> MGWGGGGGCTPRPPIHQQPPERRVVTVVFLGLLLDLLAFTLLLPLLPGLLESHGRAHDPLYGSWQGGVDWFATAIGMPVEKRYNSVLFGGLIGSAFSVLQFLCAPLTGATSDCLGRRPVMLLCLMGVATSYAVWATSRSFAAFLASRLIGGISKGNVSLSTAIVADLGSPLARSQGMAVIGVAFSLGFTLGPMLGASLPLEMAPWFALLFAASDLLFIFCFLPETLPLEKRAPSIALGFRDAADLLSPLALLRFSAVARGQDPPSGDRLSSLRRLGLVYFLYLFLFSGLEYTLSFLTHQRFQFSSLQQGKMFFLIGLTMATIQGAYARRIHPGGEVAAVKRALLLLVPAFLLIGWGRSLPVLGLGLLLYSFAAAVVVP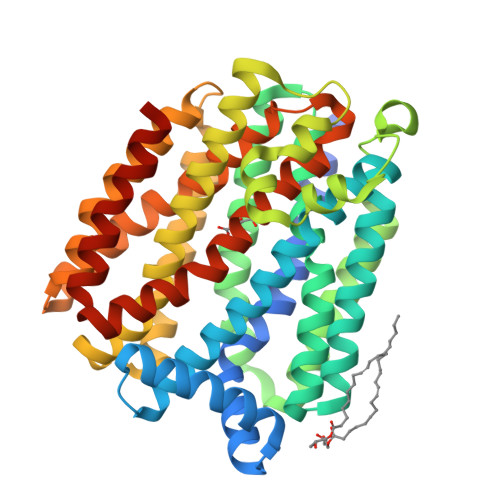CLSSVVAGYGSPGQKGTVMGTLRSLGALARAAGPLVAASVYWLAGAQACFTTWSGLFLLPFFLLQKAENLYFQ>[4x]MEGRLLLLETPGNTRMSLAYDEAIYRSFQYGDKPILRFYRHDRSVIIGYFQVAEEEVDLDYMKKNGIML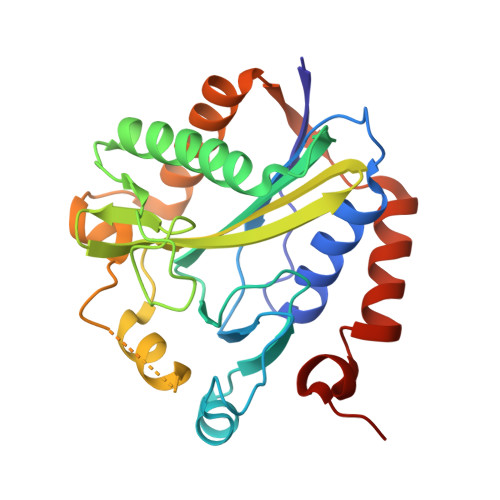ARRYTGGGAVYHDLGDLNFSVVRSSDDMDITSMFRTMNEAVVNSLRILGLDARPGELNDVSIPVNKKTDIMAGEKKIMGAAGAMRKGAKLWHAAMLVHTDLDMLSAVLKVPDEKFRDKIAKSTRERVANVTDFVDVSIDEVRNALIRGFSETLHIDFREDTITEKEESLARELFDKKYSTEEWNMGLLRKEVV>[30x]MANPTLFVSYDQNGKKLSFANWISVLSPQDTPFVSMTGKESINQTIFSWQTDALASVDGNNAHVEGSRAEDGEMKPTVIKSNVTQILRKV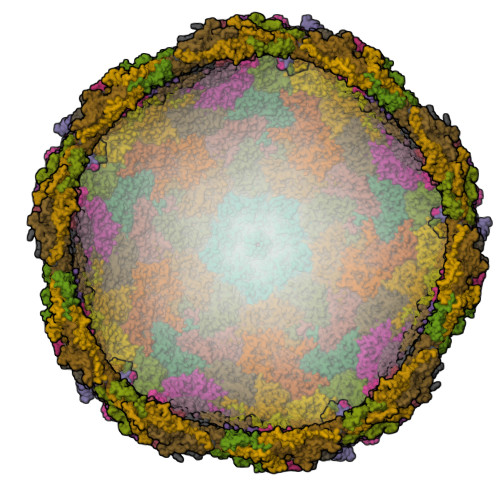VRVSDTANTTANYGRGRELMYQLEKKGKEIKRDLEKILLSGQARTDVLADQYLTNSAADPAVAGLNDTHAARKTGAFQFLCAHGGLAGGVVDKTKNGPADPDTGAVTVKVAQNASNPTTNIGFDEADIFDMTLQLYTAGSEADIIMINPAHAKIFAGLQENTQGSRKRIFENTKQFIYEVNSITDPLGQSYKIIVNRWMPTDAVYFFRSADWTQMVLRAPKRTELAKDGSYEKWMIEMEVGLRHRNPYASGVLFTAAGKAAA> GHMPRRHDPERRQRIIDAAIRVVGQKGIAGLSHRTVAAEADVPLGSTTYHFATLD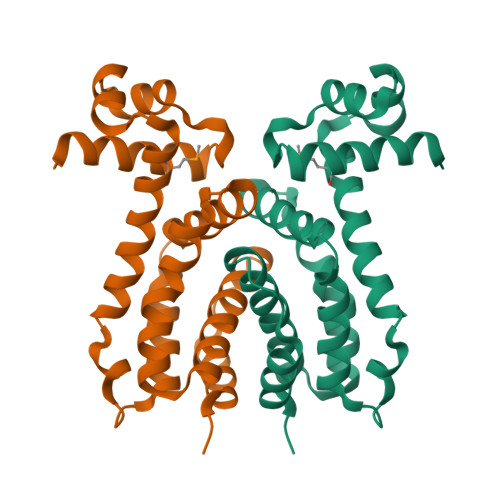DLMVAALRQANEGFARVVAAHPALSDPEADLSGELARVLGEWLGGDRTGVELEYELYLAALRRPALRPVAAEWAEGVGALLAARTDPTTARALVAVLDGICLQVLLTDTPYDEEYAREVLTRLIPVPATRDGRGPGSHPPATAGGS> RAQEDEDGDYEE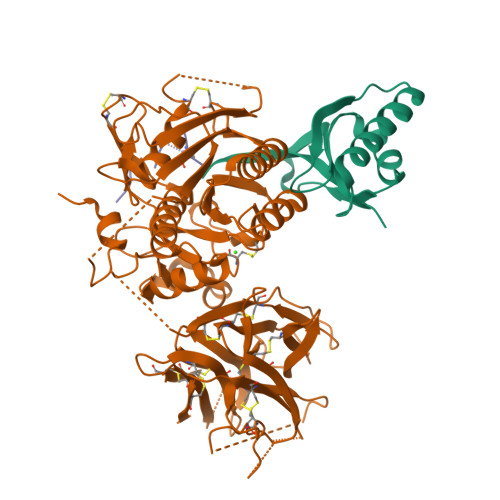LVLALRSEEDGLAEAPEHGTTATFHRCAKDPWRLPGTYVVVLKEETHLSQSERTARRLQAQAARRGYLTKILHVFHGLLPGFLVKMSGDLLELALKLPHVDYIEEDSSVFAQ;> SIPWNLERITPPRYRADEYQPPDGGSLVEVYLLDTSIQSDHREIEGRVMVTDFENVPEEDGTRFHRQASKCDSHGTHLAGVVSGRDAGVAKGASMRSLRVLNCQGKGTVSGTLIGLEFIRKSQLVQPVGPLVVLLPLAGGYSRVLNAACQRLARAGVVLVTAAGNFRDDACLYSPASAPEVITVGATNAQDQPVTLGTLGTNFGRCVDLFAPGEDIIGASSDCSTCFVSQSGTSQAAAHVAGIAAMMLSAEPELTLAELRQRLIHFSAKDVINEAWFPEDQRVLTPNLVAALPPSTHGAGWQLFCRTVWSAHSGPTRMATAIARCAPDEELLSCSSFSRSGKRRGERMEAQGGKLVCRAHNAFGGEGVYAIARCCLLPQANCSVHTAPPAEASMGTRVHCHQQGHVLTGCSSHWEVEDLGTHKPPVLRPRGQPNQCVGHREASIHASCCHAPGLECKVKEHGIPAPQEQVTVACEEGWTLTGCSALPGTSHVLGAYAVDNTCVVRSRDVSTTGSTSEEAVTAVAICCRSRHLAQASQELQHHHHHH>[2x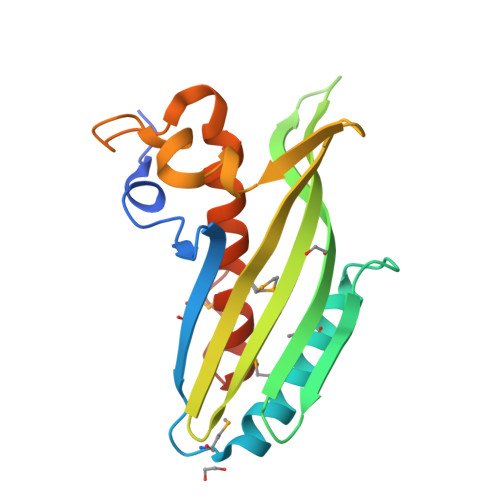]GDSAKEKKDDTRYLVGAVPEVDGKVVFSKEFQIPGMSQAQIYDTMTKWMDERLKENKNIDSRIVFSDEAKGTIAGVGEEWIVFSSSALSLDRTLVNYQITVTCKPGNCLVELEKIRFTYRETEKYKAEEWITDKYALNKAKTKLVRGLAKWRRKTVDFADDMFMDVAVAFGAPDTRPKTEK>[4x]NAKGNYCKRTPLYID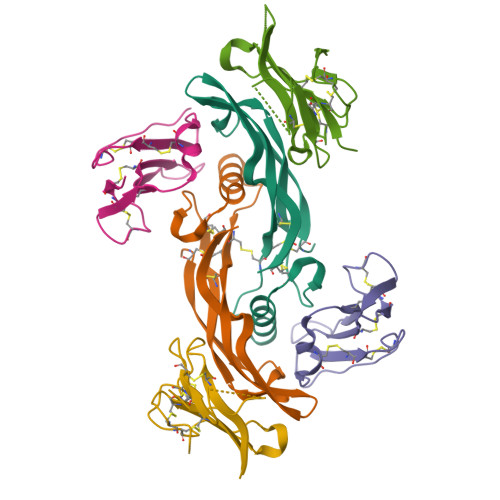FKEIGWDSWIIAPPGYEAYECRGVCNYPLAEHLTPTKHAIIQALVHLKNSQKASKACCVPTKLEPISILYLDKGVVTYKFKYEGMAVSECGCR;>DPVKPSRGPLVTCTCESPHCKGPTCRGAWCTVVLVREEGRHPQEHRGCGNLHRELCRGRPTEFVNHYCCDSHLCNHNVSLVLEATQPPSEQPGTDGQ[4x];>SQNQERLCAFKDPYQQDLGIGESRISHENGTILCSKGSTCYGLWEKSKGDINLVKQGCWSHIGDPQECHYEECVVTTTPPSIQNGTYRFCCCSTDLCNVNFTENFPPPDTTPLSPPHSFNRDET[4x]> MRTFTWRKGSLSKVNTCYVLAGGKSKRFGEDKLLYEIKGKKVIERVYETAKSVFKEVYIVAKDREKFSFLNAPVV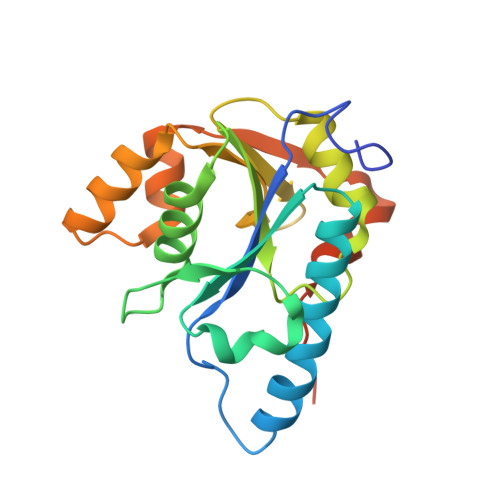LDEFEESASIIGLYTALKHAKEENVFVLSGDLPLMKKETVLYVLENFKEPVSVAKTEKLHTLVGVYSKKLLEKIEERIKKGDYRIWALLKDVGYNEVEIPEELRYTLLNMNTKEDLKRILAIENHY The nucleoprotein NP of Lassa virus, and other members of the arenavirus family, suppresses host innate immune signaling pathways, and may be linked to the profound immune disregulation noted in Lassa Fever infection. Lassa NP has a tertiary fold that is similar to, and an exonuclease active site that is completely conserved with other DEDDh exonucleases like interferon-stimulated gene-20 (ISG-20), E. coli DNA polymerase IIIε (ε186), and Trex 1 and Trex 2. Yet among this family of enzymes, Lassa NP is the only one known to have a strict specificity for a certain substrate, and the only one known to efficiently digest double-stranded RNA. The unique digestion of dsRNA by Lassa virus NP probably removes this pathogen-associated molecular pattern, and allows the virus to replicate without strong interference by the innate immune system.

Here we present the crystal structure of the exonuclease domain of Lassa NP in complex with eight bases of dsRNA. To increase the chances of obtaining a co-crystal structure of the exonuclease domain of Lassa NPΔ340 in complex with dsRNA, E391 was mutated to alanine. As a result, NPΔ340E391A is able to bind dsRNA, but cannot catalyze the exonuclease reaction to digest it. As a result of the required mutation of E391 to alanine to prevent dsRNA digestion, only one of the two cations is present in the active site in the crystal structure (site B). This site B cation is modeled as a magnesium ion, because of the presence of 5 mM MgCl2 in the crystallization buffer, and is coordinated by D389 and by one of the phosphate oxygens of the 3′ terminal nucleotide of the digested RNA strand (G8). In particular, the 2′OH of the ribose group and N2 of the nitrogenous base of G8 hydrogen bond to D426 of Lassa NP. Further, the 2′ and 3′ OH groups of G8 form hydrogen bonds to the main-chain nitrogen of G392. The ribose 2′ oxygens of C1 and C4 of the complementary, non-substrate strand (in the sequence 5′C1UCC4CUCC3′) are bound by the side chains of Q425 and D465, respectively. In addition, the nucleotide base of C1 forms a π-π interaction with Y429. The dsRNA bound to Lassa NP remains base-paired throughout the entire length, including the final residue bound into the active site.

> MAHHHHHHVDDDDRMGKPQKADSNNSSKSLQSAGFTAGLTYSQLMTLKDAMLQLDPNAKTWMDIAGRPEDPVEIALYQPSSGCYIHFFREPTDLKQFKQDAKYSHGIDVTDLFATQPGLTSAVIDALPRNMVITCQGSDDIRKLLESQGRKDIKLIDIALSKTDSRKYENAVWDQYKDLCHMHTGVVVEKKKRGGKEEITPHCALMDCIMFDAAVSGGLNTSVLRAVLPRDMVFRTSTPRVVL> MNVIAILNHMGVYFKEEPIRELHRALERLNFQIVYPNDRDDLLKLIENNARLCGVIFDWDKYNLELCEEISKMNENLPLYAFANTYSTLDVSLNDLRLQISFFEYALGAAEDIANKIKQTTDEYINTILPPLTKALFKYVREGKYTFCTPGHMGGTAFQKSPVGSLFYDFFGPNTMKSDISISVSELGSLLDHSGPHKEAEQYIARVFNADRSYMVTNGTSTANKIVGMYSAPAGSTILIDRNCHKSLTHLMMMSDVTPIYFRPTRNAYGILGGIPQSEFQHATIAKRVKETPNATWPVHAVITNSTYDGLLYNTDFIKKTLDVKSIHFDSAWVPYTNFSPIYEGKCGMSGGRVEGKVIYETQSTHKLLAAFSQASMIHVKGDVNEETFNE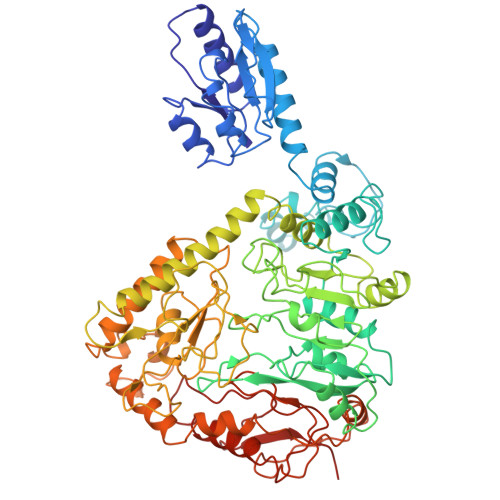AYMMHTTTSPHYGIVASTETAAAMMKGNAGKRLINGSIERAIKFRKEIKRLRTESDGWFFDVWQPDHIDTTECWPLRSDSTWHGFKNIDNEHMYLDPIKVTLLTPGMEKDGTMSDFGIPASIVAKYLDEHGIVVEKTGPYNLLFLFSIGIDKTKALSLLRALTDFKRAFDLNLRVKNMLPSLYREDPEFYENMRIQELAQNIHKLIVHHNLPDLMYRAFEVLPTMVMTPYAAFQKELHGMTEEVYLDEMVGRINANMILPYPPGVPLVMPGEMITEESRPVLEFLQMLCEIGAHYPGFETDIHGAYRQADGRYTVKVLKEESKK>MGLAPLADGEKLYGKKGSEGTVTFTKAIGDNAFVEIKT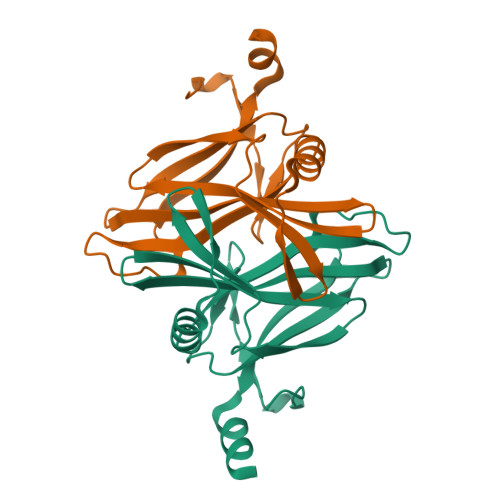GADTGFMNGCLGFSESIDGKNYWVAYVWQTKKSDTISIDMSSPVQIAEIIGTETQEVTDADTIKKLTDKIKTEKSALLQVWYASDKTGKQIDPADSASESIEVYIPSASADEALEHHHHHH[2x]>[2x]HMSFLTEEEQEAIMKVLQRDAALKRAEEERGS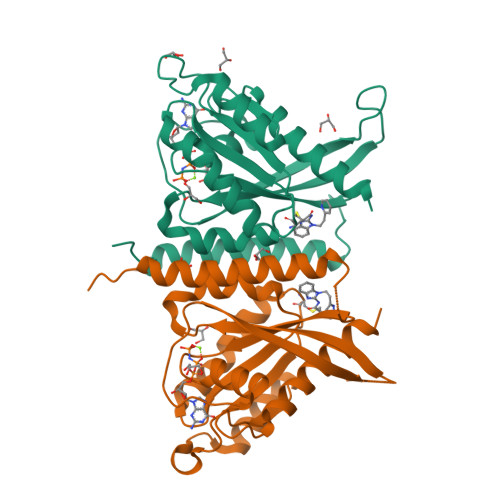GSGSGMSDGDYDYLIKFLALGDSGVGKTSVLYQYTDGKFNSKFITTVGIDFREKRVVYRASGPDGATGRGQRIHLQLWDTAGLERFRSLTTAFFRDAMGFLLLFDLTNEQSFLNVRNWISQLQMHAYCENPDIVLCGNKSDLEDQRVVKEEEAIALAEKYGIPYFETSAANGTNISQAIEMLLDLIMKRMERSVDKS>[4x]MAGDSVKSAIIGIAGGPFSGKTQLCEQLLER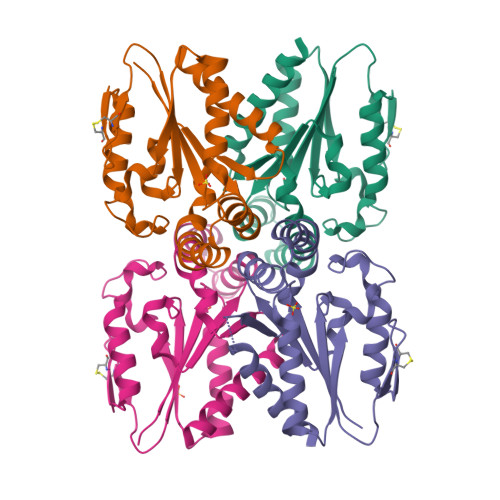LKSSAPSTFSKLIHLTSFLYPNSVDRYALSSYDIEAFKKVLSLISQGAEKICLPDGSCIKLPVDQNRIILIEGYYLLLPELLPYYTSKIFVYEDADTRLERCVLQRVKAEKGDLTKVLNDFVTLSKPAYDSSIHPTRENADIILPQKENIDTALLFVSQHLQDILAEMNKT> MEAVLNELVSVEDLLKFEKKFQSEKAAGSVSKSDQFEYAWCLVRSKYNDDIRKGIVLLEELLPKGSKEEQRDYVFYLAVGNYRL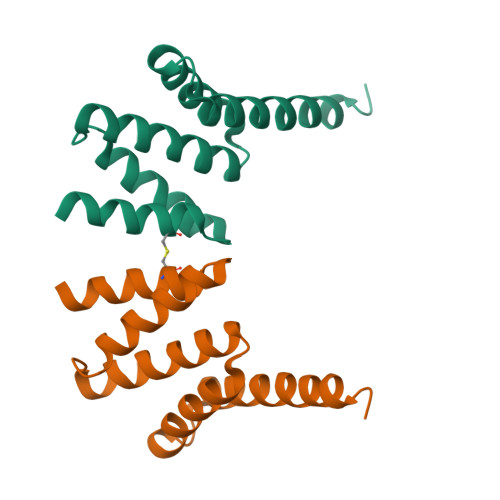KEYEKALKYVRGLLQTEPQNNQAKELERLIDKAMKKDGLLEVLFQ>[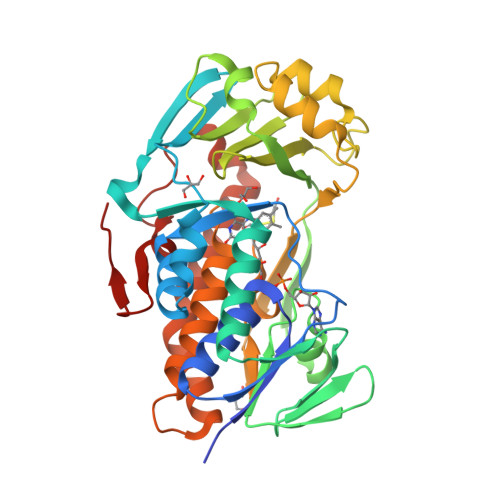2x]MANVNKTPGKTRRAEVAGGGFAGLTAAIALKQNGWDVRLHEKSSELRAFGAGIYLWHNGLRVLEGLGALDDVLQGSHTPPTYETWMHNKSVSKETFNGLPWRIMTRSHLHDALVNRARALGVDISVNSEAVAADPVGRLTLQTGEVLEADLIVGADGVGSKVRDSIGFKQDRWVSKDGLIRLIVPRMKKELGHGEWDNTIDMWNFWPRVQRILYSPCNENELYLGLMAPAADPRGSSVPIDLEVWVEMFPFLEPCLIEAAKLKTARYDKAETTKLDSWTRGKVALVGDAAHAMCPALAQGAGCAMVNAFSLSQDLEEGSSVEDALVAWETRIRPITDRCQALSGDYAANRSLSKGNMFTPAALEAARYDPLRRVYSWPQ>MNIIQGNLVGTGLKIGIVVGRFNDFITSKLLSGAEDALLRHGVDTNDIDVAWVPGAFEIPFAAKKMAETKKYDAIITLGTVIRGATTHYDYVCNEAAKGIAQAANTTGVPVIFGIVTTENIEQAIERAGTKAGNKGVDCAVSAIE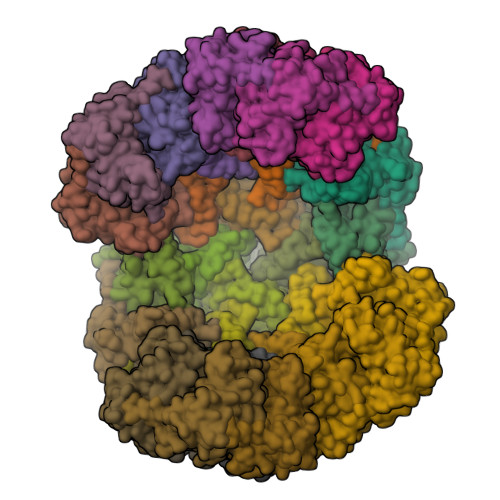MANLNRSFE[30x]> MAHHHHHHPPKRAALIQNLRDSYTETSSFAVIEEWAAGTLQEIEGIAKAAVEAHATIRNSTYGRAQAEKSPEQL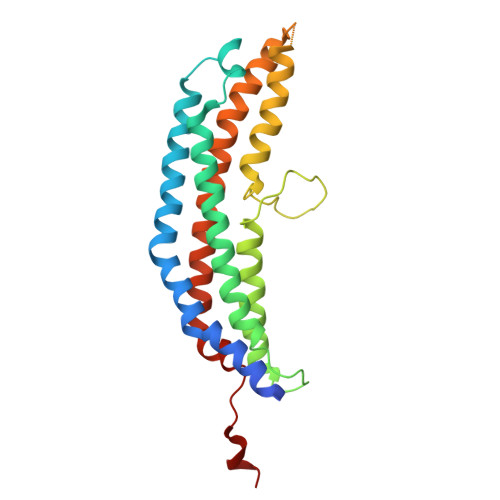LGVLQRYQDLCHNVYCQAETIRTVIAIRIPEHKEADNLGVAVQHAVLKVIDELEIKTLGSGEKSGSGGAPTPIGMYALREYLSARSTVEDKLLGSVDAESGKTKGGSQSPSLLLELRQIDADFMLKVELATTHLSTMVRAVINAYLLNWKKLIQPRGGHLDVLYR>[15x]GAPGAPGSQGAPGLQGAPGAPGSQGAPGLQGAPGAPGSQGAPGLQGAPGAPGSQGAPGLQGAPGAPGSQGAPGLQGAPGAPGSQGAPGLQGAPGAPGSQGAPGLQGAPGAPGSQGAPGLQGAPGAPGSQGAPGLQGAPGAPGSQGAPGLQGAPGAPGSQGAPGLQGAPGAPGSQGAPGLQGAPGAPGSQGAPGLQGAPGAPGSQGAPGLQGAPGAPGSQGAPGLQGAPGAPGSQGAPGLQGAPGAPGSQGAP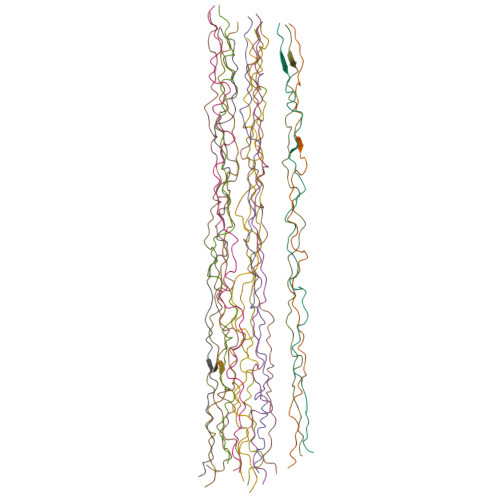GLQGAPGAPGSQGAPGLQGAPGAPGSQGAPGLQGAPGAPGSQGAPGLQGAPGAPGSQGAPGLQGAPGAPGSQGAPGLQGAPGAPGSQGAPGLQGAPGAPGSQGAPGLQGAPGAPGSQGAPGLQGAPGAPGSQGAPGLQGAPGAPGSQGAPGLQGAPGAPGSQGAPGLQGAPGAPGSQGAPGLQGAPGAPGSQGAPGLQGAPGAPGSQGAPGLQGAPGAPGSQGAPGLQGAPGAPGSQGAPGLQGAPGAPGSQGAPGLQGAPGAPGSQGAPGLQGAPGAPGSQGAPGLQGAPGAPGSQGAPGLQGAPGAPGSQGAPGLQGAPGAPGSQGAPGLQGAPGAPGSQGAPGLQGAPGAPGSQGAPGLQGAPGAPGSQGAPGLQGAPGAPGSQGAPGLQGAPGAPGSQGAPGLQGAPGAPGSQGAPGLQGAPGAPGSQGAPGLQGAPGAPGSQGAPGLQGAPGAPGSQGAPGLQGAPGAPGSQGAPGLQGAPGAPGSQGAPGLQGAPGAPGSQGAPGLQGAPGAPGSQGAPGLQ> MEAEKKKLSIPPKGIRAIIEAIRLGEIIKPSQYAKREAFKKHDVEEAWLNRVLTMIFYDIMKKQGLIDKVIKEIVGVTP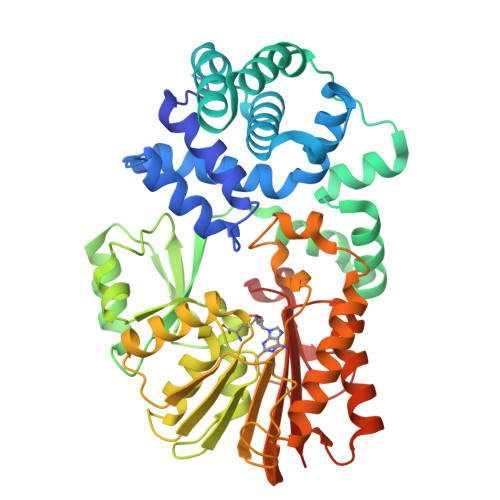LILDPWLRAALRVAVDIALFHDPSSQTIKNLRWKASDFISSRTHPYVGMYFWDLLDKIFEYKPNPKNELEELEWKYLAPSWLIERVKGILGDETEDFFRSVNKRHEWISIRVNTLKANVEEVIGELEEDGVEVVRSERVPTILKIKGPYNFDTSSAFNEGKIIVQEEASAVASIVLDPKPGETVVDLAAAPGGKTTHLAELMKNKGKIYAFDVDKMRMKRLKDFVKRMGIKIVKPLVKDARKAPEIIGEEVADKVLLDAPCTSSGTIGKNPELRWRLREDKINEMSQLQRELLESAARLVKPGGRLLYTTCSIFKEENEKNIRWFLNVHPEFKLVPLKSPYDPGFLEGTMRAWPHRHSTIGFFYALLEKSK>MEGGMKRVVLAFGTRPEATKMAPVYLALRGIPGLKPLVLLTGQHREQLRQALSLFGIQEDRNLDVMQERQALPDLAARILPQAARALKEMGADYVLVHGDTLTTFAVAWAAFLEGIPVGHVEAGLRSGNLKEPFPEEANRRLTDVLTDLDFAPTPLAKANLLKEGKREEGILVTGQTGVDAVLLAAKLGRLPEGLPEGPYVTVTMHRRENWPLLSDLAQALKRVAEAFPHLTFVYPVHLNPVVREAVFPVLKGVRNFVLLDPLEYGSMAALMRASLLLVTDSGGLQE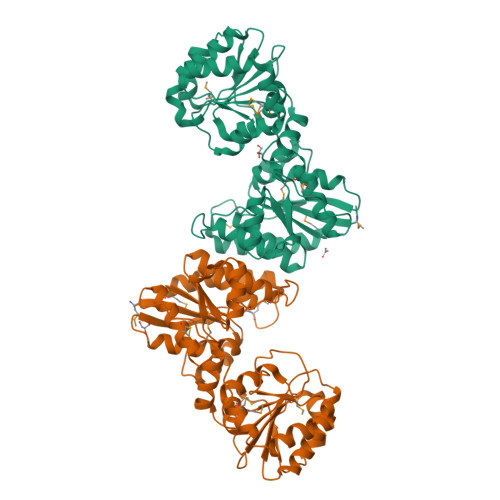EGAALGVPVVVLRNVTERPEGLKAGILKLAGTDPEGVYRVVKGLLENPEELSRMRKAKNPYGDGKAGLMVARGVAWRLGLGPRPEDWLP[2x]>GSPSSVVRDVAIIGLSGRYPQAKNVDEFWNRLKEGKNCISEIPKDRWDWQSFFDEEKGKKESMYTKWGGFIDDMDKFDPLFFQISPKEAEEMDPQERLFLQEAYASIEDAGYTPTTLCESRKVGVFVGVMNGNYPTGATYWSIANRLSYLLNFQGPSVAVDTACSASLTAIHFALESLYSGTSECAIAGGVNLIVDPVHYMKLSALTMLSPSNQCKSFGDQADGFVDGEGVGAIVLKPLDKAIADGDHIYGVIKGSMMNAGGKTNGYTVPNPQAQAQLVADALQRANVHARTVSYLEAHGTGTELGDPIEVAGLTRAFEKDTQDKQFCALGSAKSNIGHCESAAGIAGVTKILLQLKHAQLVPSLHSRTLNPNIDFTKTPFVVQQELAEWRRPIVEINGTTNEYPRIAGISSFGAGGSNAHVIIEEYIPEEQKQSSLKITPQNPAIFVLSAKNAERLYEIVQQLLAFIQEHSLSDEHLADMAYTLQVGRVAMEERIAVIAGTMKELQQKLTAYVKGQEHIADLYRGQVNRNQEMLDILTSDDELEETIARWMERGKYSKLLDLWVKGLSIDWNKLYQEEQPGRISLPTYPFAKESYWTHARSVSSSTGVGVIHPFLHQNTSDFMEQRFSSMFTGQEFFLSDHVIKGQRVLPSAAYLEMARAAIQQATGGLDSERELEGLRFKNVVWTQPLAVGPEPVQAHIELYPEANGEIVFEIYSDSKQDRDQTTEIVHSQGSAVLCSIPDIPSFDLSVLQEQCSLRTLSAEQCYDAFKKMGVDYGPAHRGIEQILIGQEQVLAKLSLPSSVVKTQGQFGLHPSLLDAALQSSLGLMMATSDFSLILPFALEEMVIVGDCSSSMWALIRYREGSKAGDRVEKFDIDLCDENGNVQVRMKGFSTRKIANVSVRSEVEVPKASVPLEEEKAIDSSSLMEQATPYFKKLLSSVIKLPANKMEADASLEKYGVDSIVAMQMTKELEKQFGSLPKTLFFEYQTIKELTGYFLENYRENLMHILGMRENAEASLTQESEATMVDEVKAQTERRSKKRKSQRFASLRMETQPPKGALDIAIIGISGRYPQARNIHDFWKNLRDGKDCITEIPKDRWDHSLYFDEAKDKLGKSYSKWGGFIDGVDQFDPLFFHISPREAELMDPQERLFLQCVYETIEDAGYTRETLGKHEGLGGNVGVYVGVMYEEYQLYASAEQALGRALAIAGSPASIANRVSYFCNFHGPSMAVDTMCSSSLTGIHLACHSLQRGECEVAIAGGVNVSIHPNKYLYLSQGKFASSKGRCESFGEGGDGYVPGEGVGAVLLKPLARAIADGDHIYGVIKGSAINHGGKTNGYTVPNPHSQSRVIRRAFEEAGIHPRTVSYIEAHGTGTSLGDPIEIAGLTKTFQEYTKENQFCAIGSAKSNIGHGESAAGIAGLTKILLQMKYKRLVPSLHSRTLNPNIDFSKTPFVVQQELAEWKRPVIEIDGVTREYARIAGISSFGAGGANAHLVIEEYIEAEHRPPSSISSKNPAVIVLSAKNKDRLREQVQRLLSAIREQVLT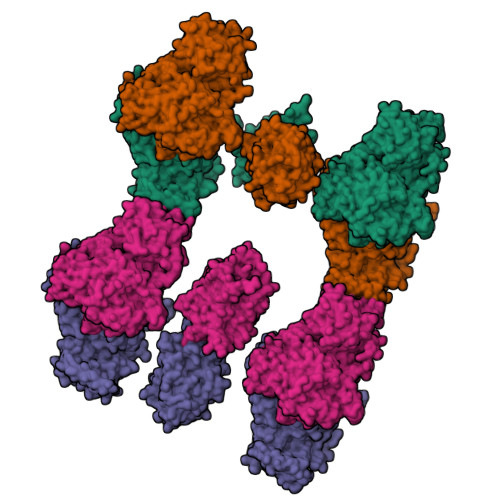DNDLAEIAYTLQVGREAMEERFAVIVKSISELEAKLTYYLKDEADSPDLFTGQVKRNKETMDVFAADEDLQQAIDTWITKGKYAKILQMWVQGLIFDWNKLYGDTKPRRISLPAYPFARERYWLPKVESQAIGLTAGEPAYLHPL[4x]>GAMTAFRIEKDTMGEVQVPADKYWAAQTERSRNNFKIGPAASMPHEIIEAFGYLKKAAAFANTDLGVLPAEKRDLIGQACDEILARKLDDQFPLVIWQTGSGTQSNMNLNEVIANRAHVINGGKLGEKSIIHPNDDVNKSQSSNDTYPTAMHIAAYKKVVEATIPAVERLQKTLAAKAAEFKDVVKIGRTHLMDATPLTLGQEFSGYAAQLSFGLTAIKNTLPHLRQLALGGTAVGTGLNTPKGYDVKVAEYIAKFTGLPFITAENKFEALATHDAIVETHGALKQVAMSLFKIANDIRLLASGPRSGIGEILIPENEPGSSIMPGKVNPTQCEAMTMVAAQVLGNDTTISFAGSQGHFELNVFKPVMAANFLQSAQLIADVCISFDEHCATGIQPNTPRIQHLLDSSLMLVTALNTHIGYENAAKIAKTAHKNGTTLREEAINLGLVSAEDFDKWVVPADMVGS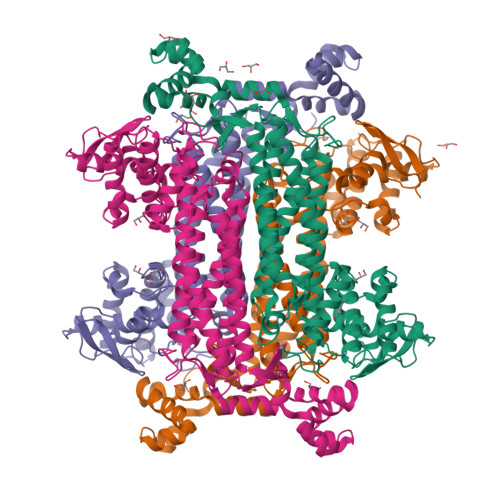LK[4x]(S)-2-AMINO-7,7-DIHYDROXYHEPTANOIC ACID | C7 H15 N O4 | 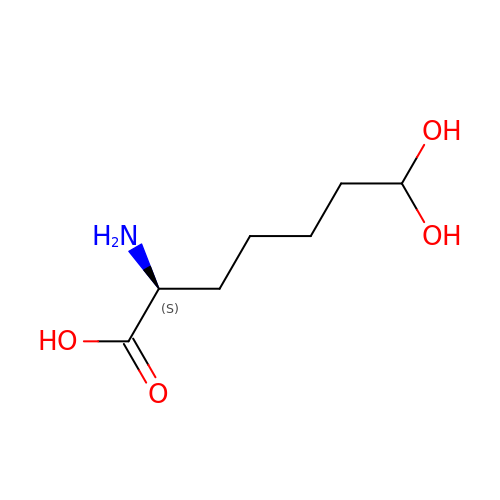KSOGSUKZGWOZJN-YFKPBYRVSA-N>MSLWRQTPDLEQLNASQKNSIGDLLGIRFEAFDDESLTASMPVDSRTHQPFGLLHGGASVVLAESLGSMASYLCVDTSQYYCVGLEVNANHLRGLRSGRVTAVARAIHLGRTTHVWDIRLSGDDGKPSCIARLTMAVVPLAGRALEHHHHH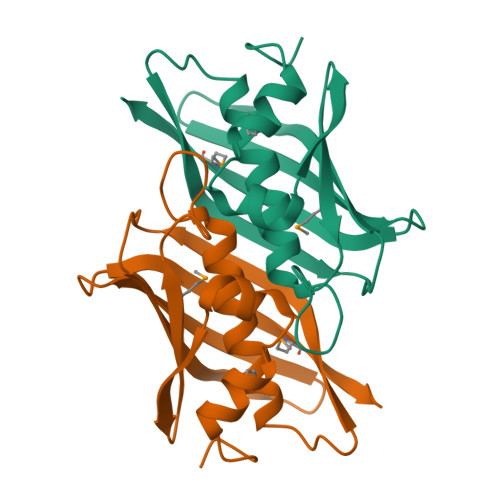H[6x]> MSKPKISLTKGKHPCTFCQARKVKCDRSLPACQNCIERNVTELCEYDDNGSRKRARLADDVNLYDKKLFNIWNQYERLWIHDTLGQCQQGVYMGIAFPLDVSEYNNTKDFYGYECLFSKESIFKILDHSLERLGWLYFGFFTDISELPYQMERYWNEYESMNINLENEEATTRQTTFKKSADQILWDLVLRSVIVMTIYYMPAKSILSLVDIDAIEKYPLDFSESNEGVDELKKKYEIFDYCLRHTLNKVLRTIFTLPPDVRTLQIFLILSNTNFLQIYPSLGNNILVHCIHLAKVLGIKDFKLKINDSGSTRLQKLSMHNIWFRLSTVDYMRSSPNKIIALHTDNSSALTRKTLFTHCSIDSIDVYDVESNLEVLRWKITSLDRDLEVSEPSLKTLKAMKELLGLLDRKTSVSNDASFNTKFESFFLKLQCNFVMWKILRYEFMQYGVTNGLQKLCCPARRIIALVANFLKEDYFEYTTHPFCVHILCVIAGFFSFYCIFHEADEVRDLRNDAVGLLKLLFDPLRPVISCFFSNLSRLEELRHIWKSVEITDQANRLVHPVMYVLKT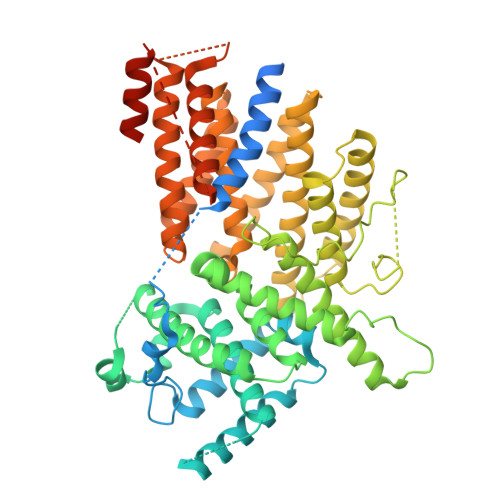DIIKLKRNLEIISGSLKDANYQETFKDKLEIDINTPALSSDFLEVVREFNLSHPLDINGKMSRQNN>MFPARLSLAVLFSVSPALAYFSGLGLGSERSIFRRDLNSTGDESNSTQWPAPLANGGKSWASAFKKAKATVTEMTVEELANITSGVIGLCSGVTGAVTRLGIPEFCLQDGPIGPRGVHGSSQFPAGLTVAATWDRTLMYARARGMGQEFHDQGVHLALAPVTGGPLGRTPLNGRGWEGTFADPYACGEASYLSVKGLTDAGVATVSKHWIAYEQETSRNLYIDIDGVSQADIQLPISSNVDDLTMHELYMWSFAEAVRAGTNHIMCSYNRINNTHSCSNAKGLNQLLKTELNFQGGVVSDWGGQWDSVPAAENGLDVAMPGKGFLGALGDFWGATLVELINNGTVSEDLVRDKAVRILTGYYYLGQDTNPPPPFVYNTIGAPTLNATSGYRNVRKPGTAELIKEIGSASVTLLKNTGSLPLKHPQRIAVLGNDATYNVLGPNACGLANSACDIDNLNGTLTTGGGSGSALSPYTITPLEALQKRAIEDNAEIAAVVANSNTTTGAEDAIAALLPDADVTFVFLNRYSEQGADAPDFSLGGDGDNLMDLAVTYSSNVVVVIHTTGVVDIEKWADNPNVTAILVAYLPGQEAGNSLVPVLYGDVAPSGKLPWTWGKSIDDYVPNGVVYTDAYSPQSNFTEGVFIDYRWFDKMGITPRYEFGFGLSYTTFTYSNLIVDHGRWAKDYSSVMETAEPFAEWDGTNSLYDVIFTVFATITNTGNLTGSEVAQLYISIPGDN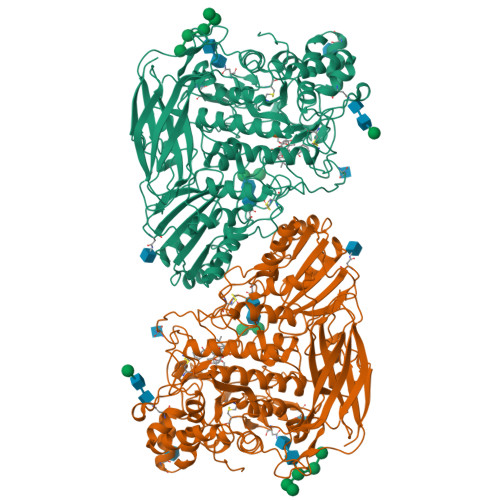QPVRQLRGFDKIKDLPVGDSAVVTFPIRRKDVSSWSVVDQLWYVPNGDFLISVGGSSRDLPLNTTWTPHHHHHH[2x]In the RAM network, the hippo-like kinase Kic1 activates the NDR-related kinase Cbk1, which forms a complex with the coactivator protein Mob2. Here we describe the crystal structure of the yeast Cbk1–Mob2 complex, providing what is to our knowledge the first structural template for an NDR/LATS kinase–Mob coactivator complex. In each structure, Mob2 binds to the conserved N-terminal extension of the Cbk1 AGC kinase domain, a region previously identified as the site by which NDR kinases bind Mob proteins. In all three structures, the Cbk1 HM peptide is wedged into a binding slot in the deep cleft formed by the kinase’s αMob helix, N-linker region, and N-terminal catalytic domain lobe.

We used two variants of catalytically inactive Cbk1(D475A) for crystallography. These differ at position 743, a highly conserved threonine and the phosphorylation site through which MST/hippo kinases (in this case, Kic1) activate NDR/LATS kinases. We collected crystallographic data on one Cbk1(HM-T)–Mob2 complex that diffracted to 3.3 Å, with one Cbk1–Mob2 complex in the asymmetric unit. Cbk1(HM-T)–Mob2 complex crystallized in only one of these states, and its substrate-binding pocket was blocked. We suggest that this is an auto-inhibited form of the kinase, while the other state seen in one of the two complexes present in Cbk1(HM-E) crystals may be competent to bind substrates containing basic amino acids (right). In our crystal structures, unphosphorylated wild-type (WT) HM region (HM-T) and HM region with glutamic acid substitution (HM-E) associate with the Mob2-supported binding site in a similar manner. Based on these data, we propose that the unphosphorylated NDR/LATS HM (HM-T) binds the kinase N-linker region, but cannot shift to a conformation that orders αC. Our structures show that there is likely an autoinhibitory HM binding site in the N-linker region, which would further hinder HM phosphorylation.

> GSSPVQSGFNNGTISNYMYFERRPDLLTKGTQDKAAAVKLKIENFYQSSVKYAIERNERRVELETELTSHNWSEERKSRQLSSLGKKESQFLRLRRTRLSLEDFHTVKVIGKGAFGEVRLVQKKDTGKIYAMKTLLKSEMYKKDQLAHVKAERDVLAGSDSPWVVSLYYSFQDAQYLYLIMEFLPGGDLMTMLIRWQLFTEDVTRFYMAECILAIETIHKLGFIHRAIKPDNILIDIRGHIKLSDFGLSTGFHKTHDSNYYKKLLQQDEATNGISKPGTYNANTTDTANKRQTMVVDSISLTMSNRQQIQTWRKSRRLMAYSTVGTPDYIAPEIFLYQGYGQECDWWSLGAIMYECLIGWPPFCSETPQETYRKIMNFEQTLQFPDDIHISYEAEDLIRRLLTHADQRLGRHGGADEIKSHPFFRGVDWNTIRQVEAPYIPKLSSITDTRFFPTDELENVPDSPAMAQAAKQREQMTKQGGSAPVKEDLPFIGYTYSRFDYLTRKNAL;> GSRNKHHSPKRHSQTSFPAQKSTPQSQQLTSTTPQSQQQEASERSESQQIMFLSEPFVRTALVKGSFKTIVQLPKYVDLGEWIALNVFEFFTNLNQFYGVVAEYVTPDAYPTMNAGPHTDYLWLDANNRQVSLPASQYIDLALTWINNKVNDKNLFPTKNGLPFPQQFSRDVQRIMVQMFRIFAHIYHHHFDKIVHLSLEAHWNSFFSHFISFAKEFKIIDRKEMAPLLPLIESFEKQGKIIYN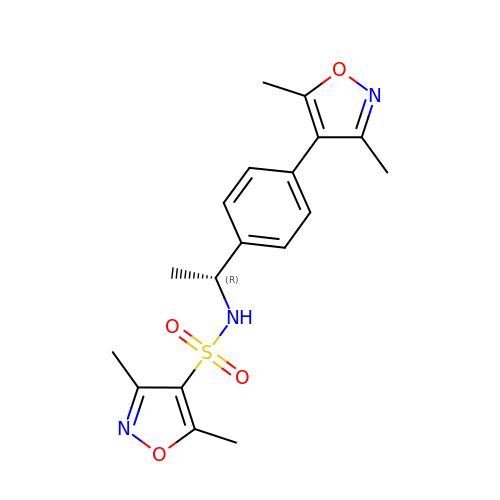(R)-N-[1-[4-(3,5-DIMETHYLISOXAZOL-4-YL)PHENYL]ETHYL]-3,5-DIMETHYLISOXAZOLE-4-SULFONAMIDE | C18 H21 N3 O4 S | QXPXDFCURRGQGI-SNVBAGLBSA-N> DYKDDDDAMGTKLEDSPPCRNWSSASELNETQEPFLNPTDYDDEEFLRYLWREYLHPKEYEWVLIAGYIIVFVVALIGNVLVCVAVWKNHHMRTVTNYFIVNLSLADVLVTITCLPATLVVDITETWFFGQSLCKVIPYLQTVSVSV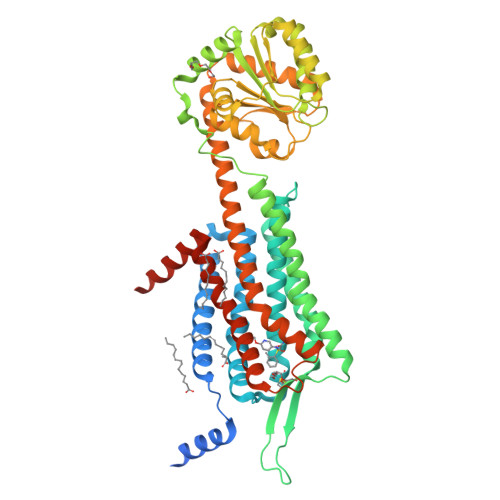SVLTLSCIALDRWYAICHPLMFKSTAKRARNSIVIIWIVSCIIMIPQAIVMECSTVFPGLANKTTLFTVCDERWGGEIYPKMYHICFFLVTYMAPLCLMVLAYLQIFRKLWCRQGIDCSFWNESYLTGSRDERKKSLLSKFGMDEGVTFMFIGRFDRGQKGVDVLLKAIEILSSKKEFQEMRFIIIGKGDPELEGWARSLEEKHGNVKVITEMLSREFVRELYGSVDFVIIPSYFEPFGLVALEAMCLGAIPIASAVGGLRDIITNETGILVKAGDPGELANAILKALELSRSDLSKFRENCKKRAMSFSKQIRARRKTARMLMVVLLVFAICYLPISILNVLKRVFGMFAHTEDRETVYAWFTFSHWLVYANSAANPIIYNFLSGKFREEFKAAFSCCCLGVHHHHHHHHHH> MSSAHNAYNAGIMQKTGKAFADEFFAEENQVVHESNAVVLVLMKSDEIDAIIEDIVLKGGKAKNPSIVVEDKAGFWWIKADGAIEIDAAEAGELLGKPFSVYDLLINVSSTVGRAYTLGTKFTITSELMGLD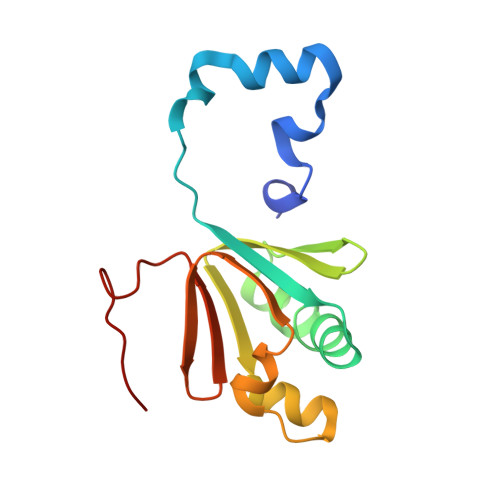RALTDI> MAEANLDKKPEVKPPPGLKAIIDHLGQVYPNQPNPLQVTTLLKYWLGGQDPLDYISMYNYPGDVDRNVPPHWHYISFGLSDLHGDERVH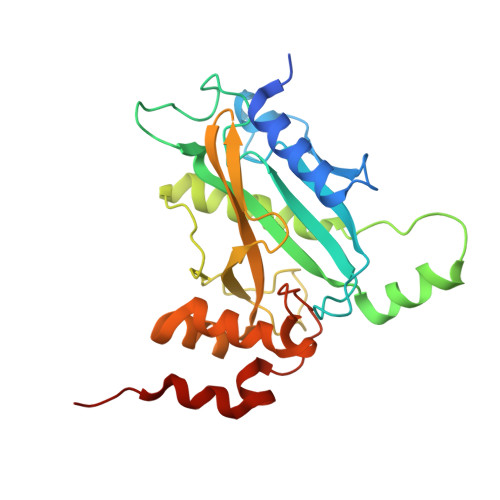LREEGVTRSGMGFELTFRLAKTEIELKQQIENPEKPQRPPTWPANLLQAIGRYCFQTGNGLCFGDNIPWRKSLDGSTTSKLQNLLVAQDPQLGCIDTPTGTVDFCQIVGVFDDELEQASRWNGRGVLNFLRQDMQTGGDWLVTNMDRQMSVFELFPETLLNLQDDLEKQ>SIQKIWAREILDSRGNPTVEVDLYTAKGLFRAAVPSGASTGIYEALELRDGDKQRYLGKGVLKAVDHINSTIAPALISSGLSVVEQEKLDNLMLELDGTENKSKFGANAILGVSLAVCKAGAAERELPLYRHIAQLAGNSDLILPVPAFNVINGGSHAGNKLAMQEFMILPVGAESFRDAMRLGAEVYHTLKGVIKDKYGKDATNVGDEGGFAPNILENSEALELVKEAIDKAGYTEKIVIGMDVAASEFYRDGKYDLDFKSPTDPSRYITGDQLGALYQDFVRDYPVVSIEDPFDQDDWAAWSKFTANVGIQIVGDDLTVTNPKRIERAVEEKACNCLLLKVNQIGSVTEAIQACKLAQENGWGVMVSHRSGETED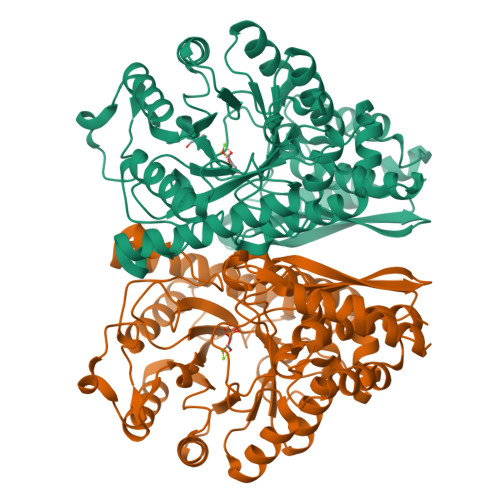TFIADLVVGLCTGQIKTGAPCRSERLAKYNQLMRIEEELGDEARFAGHNFRNPSVLHHHHHH[2x]(2S)-N-hydroxy-3-(4-methoxyphenyl)-2-[4-({[5-(pyridin-2-yl)thiophene-2-sulfonyl]amino}methyl)-1H-1,2,3-triazol-1-yl]propanamide | C22 H22 N6 O5 S2 | 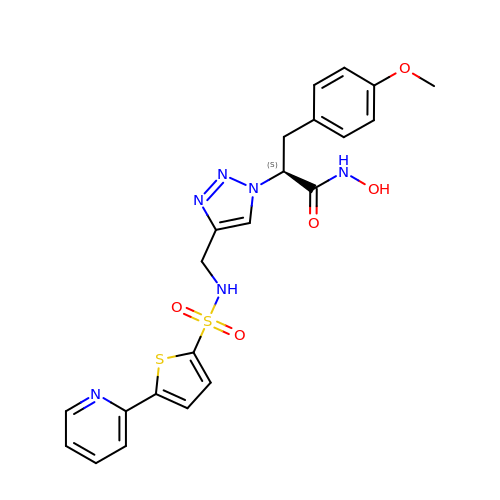VCCACZUFRCVVFN-IBGZPJMESA-N>[2x]GHMSIT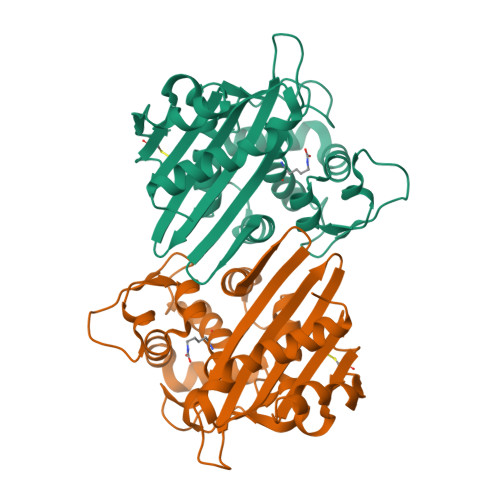ENTSWNKEFSAEAVNGVFVLCKSSSKSCATNDLARASKEYLPASTFKIPNAIIGLETGVIKNEHQVFKWDGKPRAMKQWERDLTLRGAIQVSAVPVFQQIAREVGEVRMQKYLKKFSYGNQNISGGIDKFWLEGQLRISAVNQVEFLESLYLNKLSASKENQLIVKEALVTEAAPEYLVHSKTGFSGVGTESNPGVAWWVGWVEKETEVYFFAFNMDIDNESKLPLRKSIPTKIMESEGIIG>[8x]MAGSNDVAKVMKTLD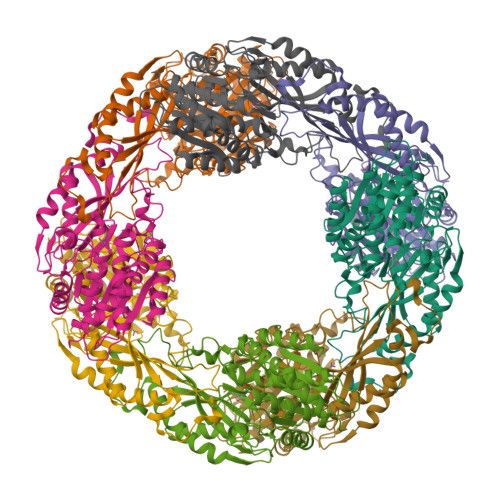GMREGLIQTAVELGSIEAPTGREGAAGDYVYEWMARNGFGPERVGVFDDRFNVVGRLRGTGGGASLSFNSHLDTIMAREDTARFADANDRIYHEAWHEEGRIYGYSVVNCKGPMACWLIAAKALKEAGAALKGDVVLTAVCGEIDCEPVDEFQGHDYLAEDIGARYAISHGAISDYALVAEATNFKPAWVEAGKVFLKVTVFAGPSRYTPYVPRPVAALDSPNAIVRMAKLVEALEEWADNYEKRYTREYGGGTVVPKVAIGAIRGGVPYKIYRFPELCSIYMDIRLNPDTNPLVVQREVEAVVSKLGLKAEVKPFLFRRGYEAQGIEPLQNALEVAHREVVGRPTERPGSPECSMWRDTNPYNELGIPSLTYGCGGGAGGGNTYFLVDDMLKAAKVYAMTAMDLCNRTP Purine nucleoside phosphorylase (PNP, purine nucleoside orthophosphate ribosyl transferase, EC 2.4.2.1) has a crucial role in the purine salvage pathway. It catalyses the reversible phosphorolytic cleavage of the glycosidic bond of purine (2′-deoxy) nucleosides, generating the corresponding free base and (2′-deoxy) ribose 1-phosphate. E. coli PNP is an excellent molecular machine conducting efficient catalysis of purine nucleosides glycosidic bond cleavage. It is a homohexamer, built as a trimer of dimers, with all its subunits having the active site in the open conformation in the apo enzyme form. Monomers in each dimer mutually donate two amino acids (His4 and Arg43) to complete their active sites.

Finally, with the highest concentrations of FA used in preparing the complexes, all the sites become occupied with FA molecules, as demonstrated by the electron density in structure DM-6(P/S)-6FA. Here all the sites clearly show the presence of the nucleoside and the refined occupancies of FA molecules are 0.7, 0.5, and 0.6 for chains A, B, and D, respectively. This is the third step in the process of FA binding to the E. coli PNP double mutant, which we could clearly identify by the X-ray crystallography method. It turned out that the conformation of both proteins with all the active sites occupied by both ligands was the same, with a closed conformation in one of three active sites. Both ligands are in the same orientation in the active sites of WT and DM, and the conformation of crucial amino acids is very similar. As already mentioned, amino acids Asp204 and Arg217 are responsible for the protonation of the nucleoside substrate. DM is not able to protonate Ado, hence its catalytic activity (maximal activity of the enzyme in the allosteric model used is 2Vmax2) is about 400-fold lower than that of WT (0.05 U mg−1 and 19.3 U mg−1, respectively).

>[3x]ATPHINAEMGDFADVVLMPGDPLRAKYIAETFLEDAREVNNVRGMLGFTGTYKGRKISVMGHGMGIPSCSIYTKELITDFGVKKIIRVGSCGAVLPHVKLRDVVIGMGACTDSKVNRIRFKDHDFAAIADFDMVRNAVDAAKALGIDARVGNLFSADLFYSPDGEMFDVMEKYGILGVEMEAAGIYGVAAEFGAKALTICTVSAHIRTHEQTTAAEAQTTFNDMIKIALESVLLGDK CHAPSO | C32 H59 N2 O8 S | 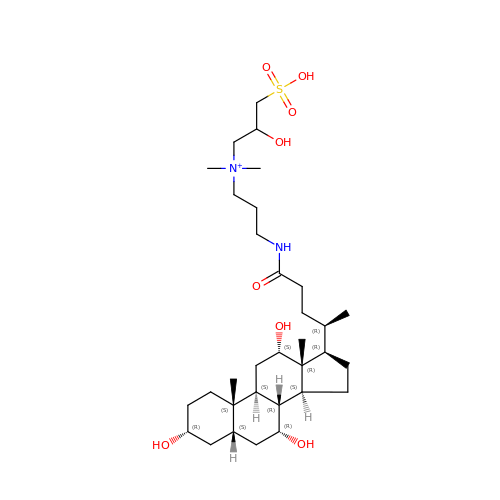GUQQBLRVXOUDTN-XOHPMCGNSA-O>SFGRDACSEMSIDGLCQCAPIMSEYEIICPANAENPTFRLTIQPKDYVQIMCNLTDTTDYQQLPKKLRIGEVDRVQMRRCMLPGHTPIASILDYLGIVSPTTLIFESDNLGMNITRQHLDRLHGLKRFRFTTRRLTHIPANLLTDMRNLSHLELRANIEEMPSHLFDDLENLESIEFGSNKLRQMPRGIFGKMPKLKQLNLASNQLKSVPDGI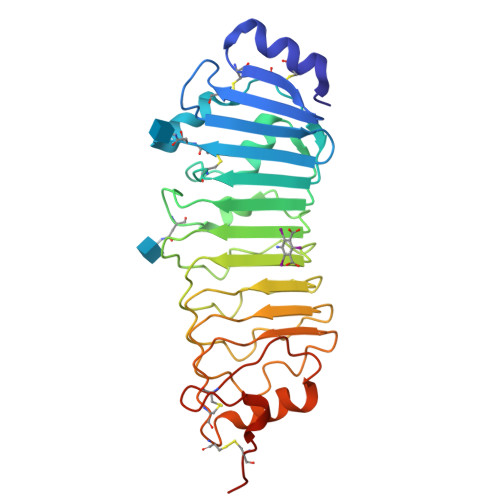FDRLTSLQKIWLHTNPWDCSCPRIDYLSRWLNKNSQKEQGSAKCSGSGKPVRSIICPTTGENLYFQ[2x]> GPLGSPEFPGRRKPEAQPFAHLTINAASIPSGSHKVTLSSWYHDRGWAKISNMTLSNGKLRVNQDGFYYLYANICFRHHETSGSVPTDYLQLMVYVVKTSIKIPSSHNLMKGGSTKNWSGNSEFHFYSINVGGFFKLRAGEEISIQVSNPSLLDPDQDAT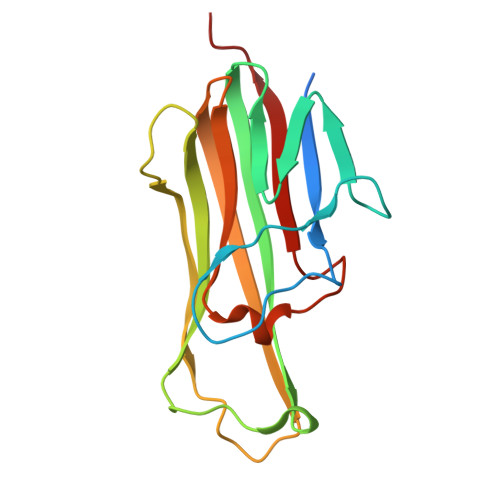YFGAFKVQDID> SMYFQSMLSLTLLGAAVVGQECEVQIVFKNPLPVTLTNVVFRLEGSGLQRPKILNVGDIGGNETVTLRQSFVPVRPGPRQLIASLDSPQLSQVHGVIQVD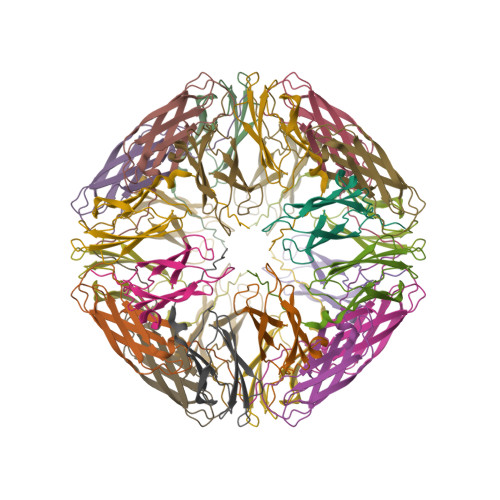VA>MMGYIPYVIENTDRGERSYDIYSRLLKDRIVLLSGEINDSVASSIVAQLLFLEAEDPEKDIGLYINSPGGVITSGLSIYDTMNFIRPDVSTICIGQAASMGAFLLSCGAKGKRFSLPHSRIMIHQPLGGAQGQASDIEIISNEILRLKGLMNSILAQNSGQSLEQIAKDTDRDFYMSAKEAKEYGLIDKVLQKNVK[14x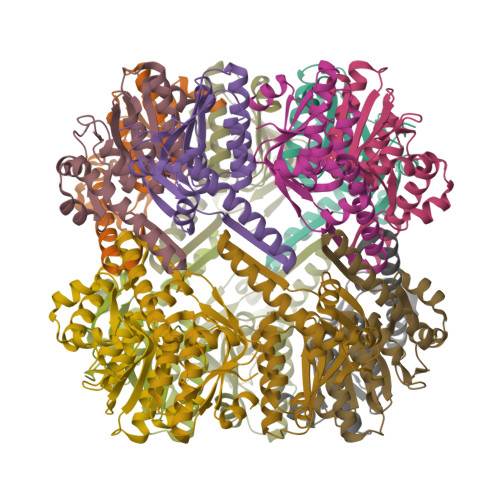]> SMEILQVALHKRDSGEQLGIKLVRRTDEPGVFILDL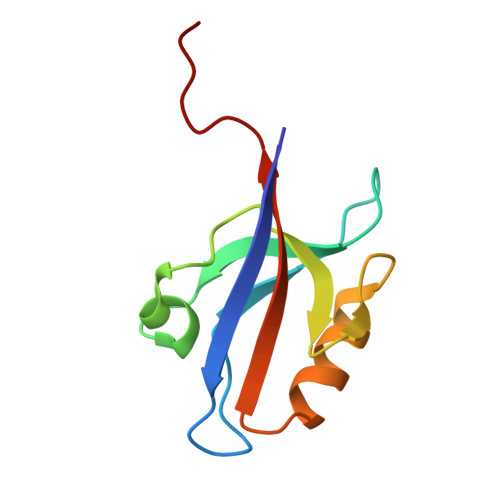LEGGLAAQDGRLSSNDRVLAINGHDLKYGTPELAAQIIQASGERVNLTIARPGKPEIEL>AAIVPTRELENVFLGRCKDYEITRYLDILPRVRSDCSALWKDFFKAFSFKNPCDLDLGSYKDFFTSAQQQLPKNKVMFWSGVYDEAHDYANTGRKYITLEDTLPGYMLNSLVWCGQRANPGFNEKVCPDFKTCPVQARESFWGMASSSYAHSAEGEVTY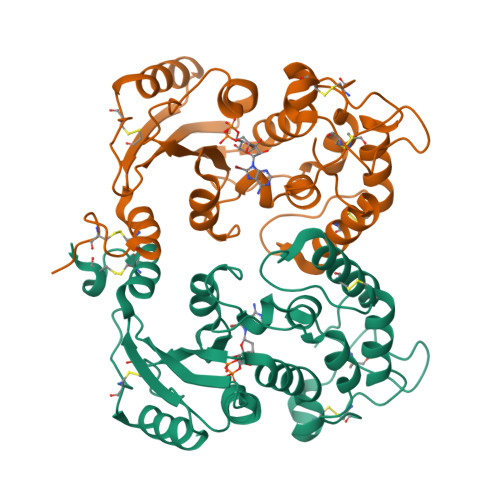MVDGSNPKVPAYRPDSFFGKYELPNLTNKVTRVKVIVLHRLGEKIIEKCGAGSLLDLEKLVKAKHFAFDCVENPRAVLFLLCSDNPNARECRLAKRFYRIA[8x]> MSAEGYQYRALYDYKKEREEDIDLHLGDILTVNKGSLVALGFSDGQEARPEEIGWLNGYNETTGER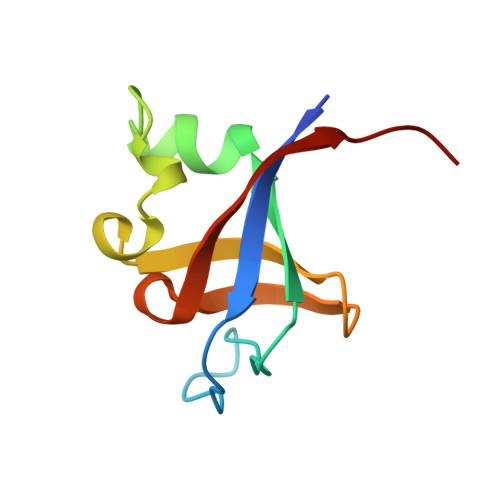GDFPGTYVEYIGRKKISPP>[4x]SNAMSEKIAFLGLGNLGTPIAEILLEAGYELVVWNRTASKAEPLTKLGATVVENAIDAITPGGIVFSVLADDAAVEELFSMELVEKLGKDGVHVSMSTISPETSRQLAQVHEWYGAHYVGAPIFARPEAVRAKVGNICLSGNAGAKERIKPIVENFVKGVFDFGDDPGAANVIKLAGNFMIACSLEMMGEAFTMAEKNGISRQSIYEMLTSTLFAAPIFQNYGKL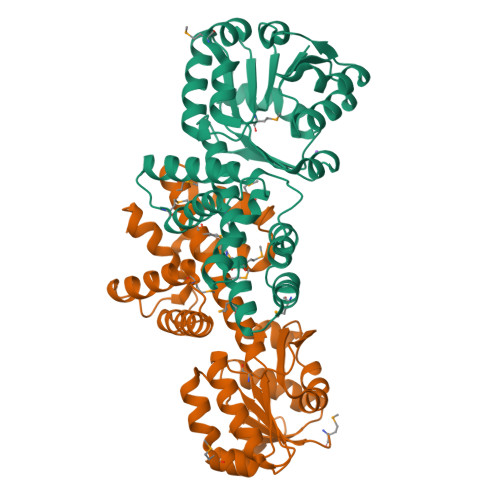VASNTYEPVAFRFPLGLKDINLTLQTASDVNAPMPFADIIRNRFISGLAKGRENLDWGALALGASDDAGLTK>MTYGGRDQQYNKTNYKSRGGDFRGGRNSDRNSYNDRPQGGNYRGGFGGRSNYNQPQELIKPNWDEELPKLPTFEKNFYVEHESVRDRSDSEIAQFRKENEMTISGHDIPKPITTFDEAGFPDYVLNEVKAEGFDKPTGIQCQGWPMALSGRDMVGIAATGSGKTLSYCLPGIVHINAQPLLAPGDGPIVLVLAPTRELAVQIQTECSKFGHSSRIRNTCVYGGVPKSQQIRDLSRGSEIVIATPGRLIDMLEIGKTNLKRVTYLVLDEADRMLDMGFEPQIRKIVDQIRPDRQTLMWSATWPKEVKQLAADYLNDPIQVQVGSLELSASHNITQIVEVVSDFEKRDRLNKYLET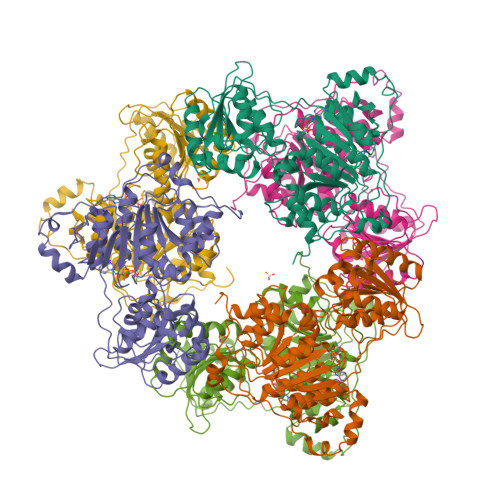ASQDNEYKTLIFASTKRMCDDITKYLREDGWPALAIHGDKDQRERDWVLQEFRNGRSPIMVATDVAARGIDVKGINYVINYDMPGNIEDYVHRIGRTGRAGATGTAISFFTEQNKGLGAKLISIMREANQNIPPELLKYDRRSYGGGHPRYGGGRGGRGGYGRRGGYGGGRGGYGGNRQRDGGWGNRGRSNY[6x]> 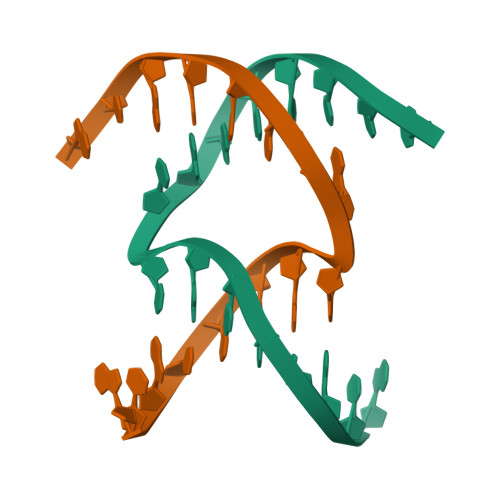GTACCAGCCGAACCTG;> ACGCTGGTGGTTCGCA> MSMNIYVGNLNYRVREEDLTGLLQQYGAVTSARVITDRETGRSRGFGFVEMEDENDARR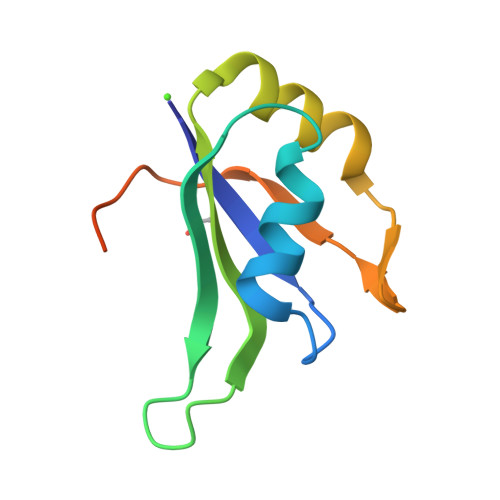AIEELFDQEFQGRKLIVKEALERPERAPRRTFRHEDRY> CGFGGSGSNGEGKKDSKGKTTLNINIKTEPFSLHPGLANDSVSGGVIRQTFEGLTRINADGEPEEGMASKIETSKDGKTYTFTIRDGVKWSNGDPVTAQDFEYAWKWALDPNNESQYAYQLYYIKGAEAANTGKGSLDDVAVKAVNDKTLKVELNNPTPYFTELTAFYTYMPINKKIAEKNKKWNTNAGDDYVSNGPFKMTAWKHSGSITLEKNDQYWDKDKVKLKKIDMVMINNNNTELKKFQAGELDWAGMPLGQLPTESLPTLKKDGSLHVEPIAGVYWYKFNTEAKPLDNVNIRKALTYSLDRQSIVKNVTQGEQIPAMAAVPPTMKGFEDNKEGYFKDNDVKT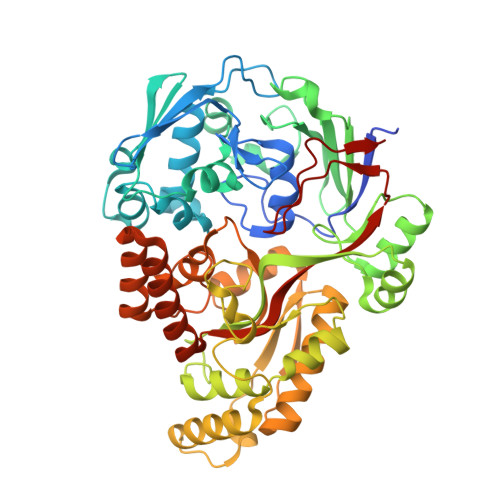AKEYLEKGLKEMGLSKASDLPKIKLSYNTDDAHAKIAQAVQEMWKKNLGVDVELDNSEWNVYIDKLHSQDYQIGRMGWLGDFNDPINFLELFRDKNGGNNDTGWENPEFKKLLNQSQTETDKTKRAELLKKAEGIFIDEMPVAPIYFYTDTWVQDENLKGVIMPGTGEVYFRNAYFK>[2x]GGCGACUG;>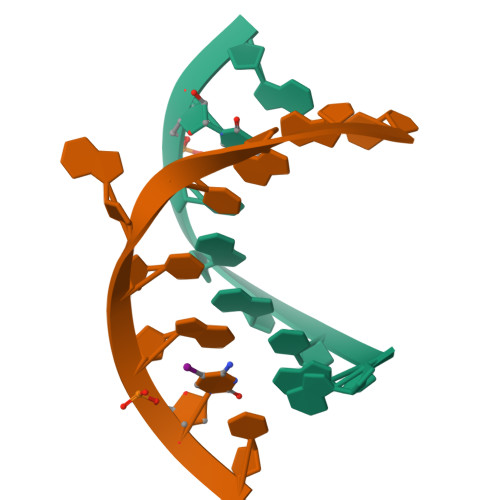[2x]CAGUACGCC> MITDCFEADIAIPSGISRPDAAALQRCEGRVVFLPTIRRQLA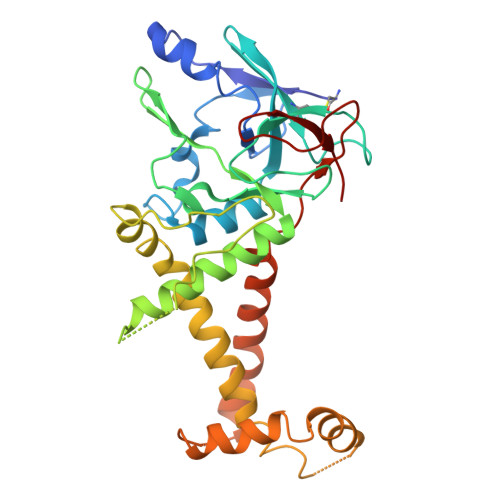LADVAHESFVSGGVSPDTLGLLLAYRRRFPAVITRVLPTRIVACPVDLGLTHAGTVNLRNTSPVDLCNGDPVSLVPPVFEGQATDVRLESLDLTLRFPVPLPTPLAREIVARLVARGIRDLNPDPRTPGELPDLNVLYYNGARLSLVADVQQLASVNTELRSLVLNMVYSITEGTTLILTLIPRLLALSAQDGYVNALLQMQSVTREAAQLIHPEAPMLMQDGERRLPLYEALVAWLAHAGQLGDILALAPAVRVCTFDGAAVVQSGDMAPVIRYP>[4x]GSNMKAVCVMTGTAGVKG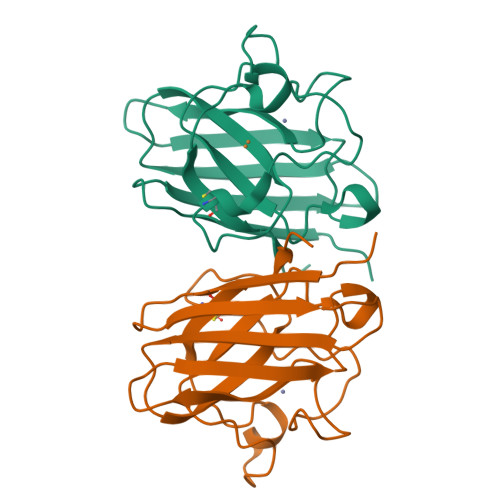VVKFTQETDNGPVHVHAEFSGLKAGKHGFHVHEFGDTTNGCTSAGAHFNPTKQEHGAPEDSIRHVGDLGNVVAGADGNAVYNATDKLISLNGSHSIIGRSMVIHENEDDLGRGGHELSKVTGNAGGRLACGVVGLAAE> ETGSIVLEPIYWNSSNSKFLPGQGLVLYPQIGDKLDIICPKVDSKTVGQYEYYKVYMVDKDQADRCTIKKENTPLLNCAKPDQDIKFTIKFQEFSPNLWGLEFQKNKDYY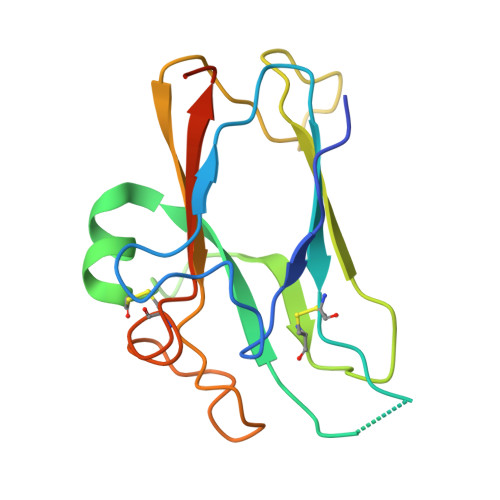IISTSNGSLEGLDNQEGGVCQTRAMKILMKVGQDGTKHHHHHH> AA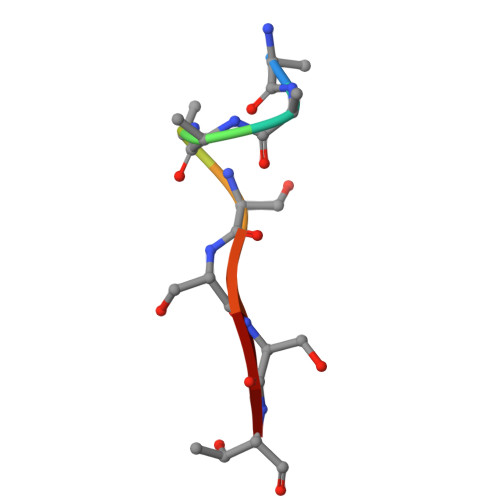AASSST> MVKQIESKTAFQEALDAAGDKLVVVDFSATWCGPCKMIKPFFHSLSEKYSNVIFLEVDVNDCQDVASE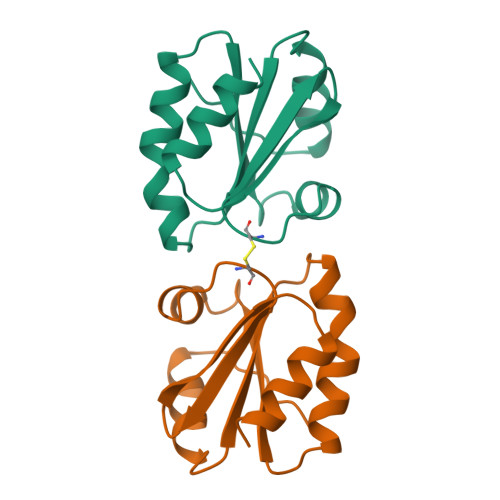CEVKCMPTFQFFKKGQKVGEFSGANKEKLEATINELV>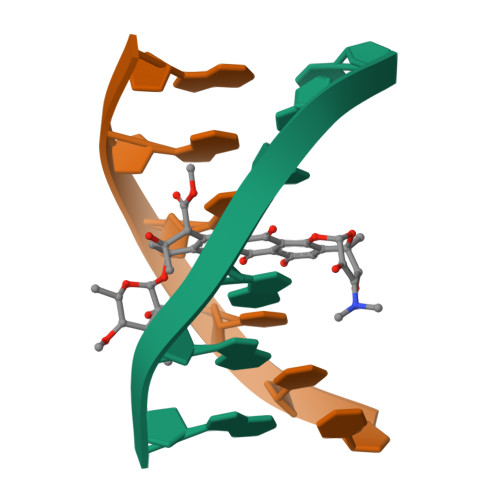CCCGGG[2x]>[4x]MKFSKGIHAIDSHTMGEPTRIVVGGIPQINGETMADKKKYLEDNLDYVRTALM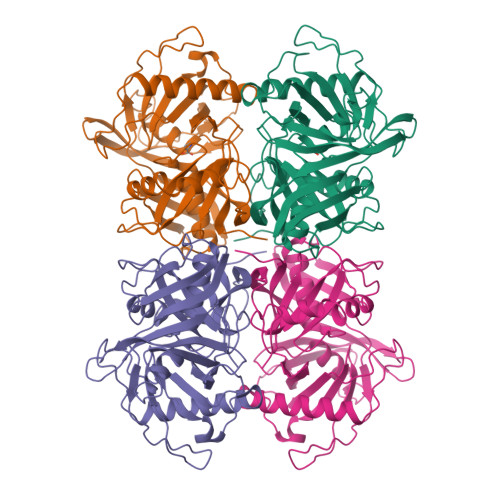HEPRGHNDMFGSIITSSNNKEADFGIIFMDGGGYLNMCGHGSIGAATVAVETGMVEMVEPVTNINMEAPAGLIKAKVMVENEKVKEVSITNVPSFLYMEDAKLEVPSLNKTITFDISFGGSFFAIIHAKELGVKVETSQVDVLKKLGIEIRDLINEKIKVQHPELEHIKTVDLVEIYDEPSNPEATYKNVVIFGQGQVDRSPCGTGTSAKLATLYKKGHLKIDEKFVYESITGTMFKGRVLEETKVGEFDAIIPEITGGAYITGFNHFVIDPEDPLKYGFTVLEHHHHHH>GPGSLSTNHETIDLLVQILRNCLRYFLPPSFPISKKQLSAMNSDELISFPLKEYFKQYEVGLQN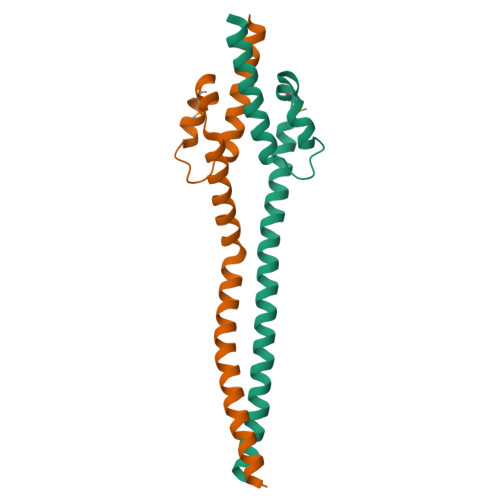LCNSYQSRADSRAKASEESLRTSERKLRETEEKLQKLRTNIVA[2x]> PESELIRQSWRVVSRSPLEHGTVLFARLFALEPSLLPLFQYNGRQFSSPEDSLSSPEFLDHIRKVMLVIDAAVTNVEDLSSLEEYLTSLGRKHRAVGVRLSSASTVGESLLYMLEKSLGPDFTPATRTAWSRLYGAVVQAMSRGWD

Ngb is over-expressed in hypoxic conditions and it may be involved in gas/redox sensing, radical scavenging, and/or signal transduction. Notably, hexacoordination in Ngb accounts for a peculiar structural rearrangement and complex kinetics upon ligand binding, which takes place when the distal histidine (His(E7)64), engaged in internal iron hexacoordination, dissociates from the heme. The dissociation of His64 is the rate-limiting step for ligand binding and it triggers a repositioning of the heme which slides further inside a large internal cavity. In this study, we spectroscopically and structurally characterized three Ngb mutants aiming at pinpointing key features: a CD loop mutant with enhanced flexibility (Gly-loop), the F106A mutant and the double Gly-loop/F106A mutant.

Crystal structures of unliganded hexacoordinated F106A (1.8 Å) and carbomonoxy-F106A (F106A-CO, 1.75 Å), were determined to observe the effect of removal of the steric barrier to heme sliding posed by Phe106. At this resolution, we clearly detect the double heme conformation: the B conformer (canonical, 30% in ferric F106A, 27% in F106A-CO) and the A one (reversed, 70% in ferric F106A, 73% in F106A-CO). As compared to WT Ngb, the structural difference between the two conformers is larger, likely due to the wider heme cavity, created by the Phe to Ala substitution that allows conformer B to adopt a deeper position within the pocket. We also observed double conformations for proximal and distal histidines. The geometry of the His64-Fe-His96 bond, for both conformers, appears to be different with respect to WT Ngb and it might contribute to reactivity with ligands. However, the most striking observation about heme conformations is the relative position of the A and B conformers, that are laterally and vertically shifted, with their iron atoms being about 1.0 Å and 0.90 Å apart, respectively in the unliganded and in the carbomonoxy form. Consistently, Phe(CD1)42, a conserved residue involved in the heme packing through π-π stacking interactions, adopts a double conformation in a 70:30 proportion (lateral displacement of 1.0 Å at the level of Phe42 Cζ, not shown) in the structure of unliganded F106A. The effect of the double heme insertion observed in Ngb is enhanced by the increased size of the large Ngb internal cavity created by the F106A mutation, which results in a set of alternate conformations of proximal side residues that account for the enhanced biphasic behaviour in ligand binding of mutants carrying this substitution.>GHMAIPKLQAYALPESHDIPQNKVDWAFEPQRAALLIHDMQDYFVSFWGENCPMMEQVIANIAALRDYCKQHNIPVYYTAQPKEQSDEDRALLNDMWGPGLTRSPEQQKVVDRLTPDADDTVLVKWRYSAFHRSPLEQMLKESGRNQLIITGVYAHIGCMTTATDAFMRDIKPFMVADALADFSRDEHLMSLKYVAGRSGRVVMTEELLPAPIPASKAALREVILPLLDESDEPFDDDNLIDYGLDSVRM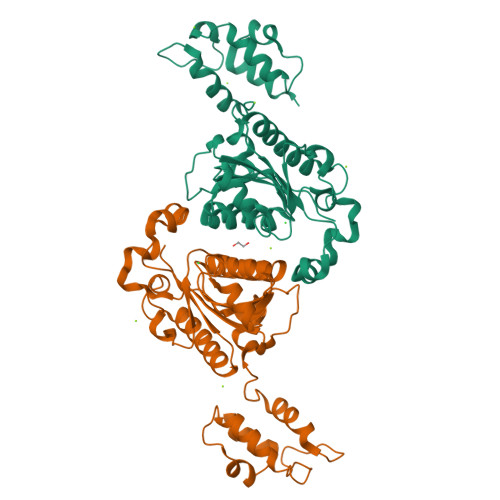MALAARWRKVHGDIDFVMLAKNPTIDAWWKLLSREVK[2x]Shy (side chain hydratase) and Sal (side chain aldolase), are involved in successive reactions in the pathway of bile acid side chain catabolism in Proteobacteria. In contrast, the hydratase, Shy, (side chain hydratase) thought to be responsible for a similar reaction in Proteobacteria, contains a single MaoC domain possessing the His/Asp catalytic dyad in the C terminus and a DUF35 domain in the N terminus. We showed that this aldolase, Sal, forms a complex with the hydratase, Shy, that catalyzes the preceding reaction. Shy contains a MaoC domain and a DUF35 domain, the latter which is responsible for interaction with Sal.

The crystal structure of ShyMaoC was determined to 2.05 Å resolution by molecular replacement using a protomeric model of the protein as predicted by ColabFold as the search model. Although the crystal was grown in the presence of acetyl CoA, electron density for the ligand was not observed in the structure. ShyMaoC crystallizes with two chains in the asymmetric unit; these protomers superimpose closely with an r.m.sd of 0.3 Å. ShyMaoC adopts a hot dog fold, with a central bent five-stranded antiparallel β-sheet (topology 2, −5, 6, −7, 4) “bun” wrapping around a central helix “sausage”, inserted between β2 and β3. The two ShyMaoC protomers interact to form a homodimer with an interface area of 1001.9 Å2 (as determined by proteins, interfaces, structures and assemblies, PISA). β4 strands from adjacent protomers interact in antiparallel fashion to form an extended 10-strand β-sheet; in addition, the central helix, α5, and α4 from the active site housing of each protomer interact to form a four-helix bundle which buries an extended nonpolar surface. Firstly, the central helix of ShyMaoC is only nine residues long, with the shortening of the helix by an additional turn at the C terminal (relative to the already shortened PaaZMaoC) opening up considerable additional space in the active site. The loop C terminal to this central helix is also greatly elongated, forming β3 of the auxiliary domain before linking back to β4 of the central β-sheet; this pushes these residues to the periphery of the binding site, where they form an extended wall of an open pocket rather than forming one side of the substrate binding tunnel. The active site is further opened up by a small shift outward of the active site housing; as a result of this shift (along with the shortening of the central helix and the α5-β3 loop) α3 and α4 do not make contact with the dimeric partner. Together these changes produce a continuous open cleft that spans the width of the β-sheet with an approximate volume of 2895 Å3. The steroid nucleus packs across the β-sheet, interacting with an extended hydrophobic patch comprised of the side chains of Met-289 and Leu-291 on β5, Leu-307 and Ile-309 on β6, and Met-249 on β4.

>[2x]KRRISVKDIEAMKSLVSEEYSPWSNEFTVSQEVIDEFARLSGDDYWIHTDPVQAREKSPFGTTIAHGALVQVLASQLRIPLDYEVVDFNNMVNYGSDRLRFPTPVPSGCKIRARARIKAVEQVRSGVQATMELNIHVVGQDRPAVINDLVILYM> PELPEVETIRRTLLPLIVGKTIEDVRIFWPNIIRHPRDSEAFAARMIGQTVRGLERRGKFLKFLLDRDALISHLRAEGRYAVASALEPLEPHTHVVFCFTDGSELRYRDVRKFGTMHVYAKEEADRRPPLAELGPEPLSPAFSPAVLAERAVKTKRSVKALLLDCTVVAGFGNIY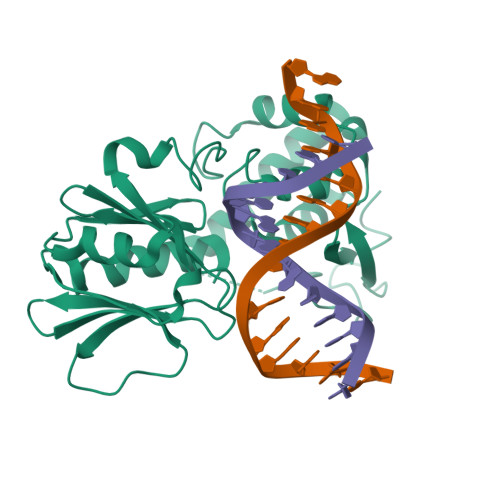VDESLFRAGILPGRPAASLSSKEIERLHEEMVATIGEAVMKGGSTVRTYVNTQGEAGTFQHHLYVYGRQGNPCKRCGTPIEKTVVAGRGTHYCPRCQR>MRIPLVGKDSIESKDIGFTLIHEHLRVFSEAVRQQWPHLYNEDEEFRNAVNEVKRAMQFGVKTIVDPTVMGLGRDIRFMEKVVKATGINLVAGTGIYIYIDLPFYFLNRSIDEIADLFIHDIKEGIQGTLNKAGFVKIAADEPGITKDVEKVIRAAAIANKETKVPIITHSNAHNNTGLEQQRILTEEGVDPGKILIGHLGDTDNIDYIKKIADKGSFIGLDRYGLDLFLPVDKRNETTLRLIKDGYSDKIMISHDYCCTIDTGTAKPEYKPKLAPRWSITLIFEDTIPFLKRNGVNEEVIATIFKENPKKFFS[4x]

PLLs are natural lactonases endowed with promiscuous phosphotriesterase activity. The catalytic center contained two metal cations coordinated by four histidines, an aspartic acid and a carboxylated lysine residue. A structural analysis of SsoPox, a hyperthermostable counterpart of the PLL family from Sulfolobus solfataricus, has revealed that loop 7 is shorter in SsoPox than in PTEs; linking the active site to the loop 8, which forms a hydrophobic channel that accommodates AHLs aliphatic chain. Indeed, W263 is located at the start of loop 8, involved in the dimer interface of the enzyme and positions the lactone cycle of the substrate onto the bi-metallic catalytic center.

A single mutation of W263 can significantly increase the paraoxonase activity of the enzyme (by 23-fold with the W263F substitution), the oxo-lactonase activity (by 148-fold with the W263T substitution) and the activity toward the poor AHL substrate (3-oxo-C12 AHL; by 55-fold (W263V)). However, whereas detergent-induced flexibility has no effect on the lactonase activity, we isolated variants of W263 that exhibit increased lactonase activities (W263T/V/I). These variants exhibit dramatic improvement of their oxo-lactonase catalytic efficiencies (148-fold for variant W263T), while the activity for the best AHL substrate is compromised (3-oxo-C10 AHL; for the wild-type enzyme). Conversely, the LacSV group dramatically increases oxo-lactonase activity and 3-oxo-C12 AHLase activities, while the phosphotriesterase activity is mildly modulated and 3-oxo-C10 AHLase is decreased. The residues selected in the LacSV group (T, V, I) are overall smaller than those selected in the PteSV group (F, L, M) with the exception of isoleucine (I). Mutations W263V-T therefore yield enlarged active site cavities for the lactone variants. On the contrary, the paraoxonase activity of LacSV variants exhibit a behavior that is similar to that of the wild-type enzyme, i.e., the activity keeps increasing with temperature (or remains higher than ambient temperature activity for W236T around its Tm). The analysis of the normalized B-factors of the variants clearly reveal that the substitution W263 is destabilizing (as confirmed by the Tm of the variants), but also that the active site loops of PteSV are significantly more disordered than those of LacSV. PteSV lose their activity before the loss of the global structure (Tm), whereas LacSV do not, and exhibit a similar thermophilicity profile to that of the wild-type enzyme.>[3x]GMYNPVGVAAIGLGRWAYVMADAYTKSEKLKLVTCYSRTEDKREKFGKRYNCAGDATMEALLAREDVEMVIITVPNDKHAEVIEQCARSGKHIYVEKPISVSLDHAQRIDQVIKETGVKFLCGHSSRRL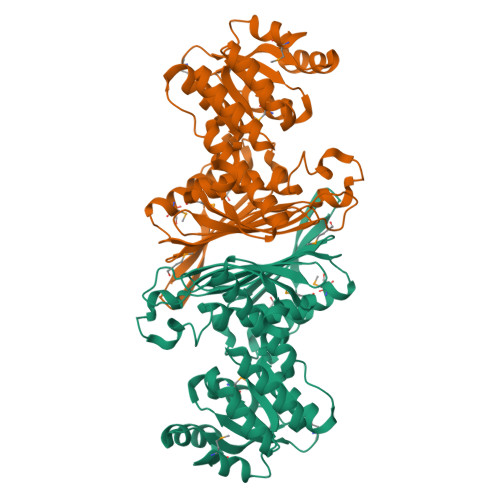GALRKMKEMIDTKEIGEVSSIEAVFSNERGLELKKGNWRGEPATAPGGPLTQLGVHQIDNLQFLLGPVARVFNFGKPMYTEVENITVNQTLLEFEDGKQAYLGTNWACPGVFSINVYGTKANLFYQLDFSWWSNSDVTDEHSTLIKREFASMSDDPDNRILRDVKVDFESVDHLRVEVEEVADVIRNGGETEIGAEASLRNLAVVLAAVKSVHEKRPVEIAEIIG>AEEFPVPNGFESAYREVDGVKLHYVKGGQGPLVMLVHGFGQTWYEWHQLMPELAKRFTVIAPDLPGLGQSEPPKTGYSGEQVAVYLHKLARQFSPDRPFDLVAHDIGIWNTYPMVVKNQADIARLVYMEAPIPDARIYRFPAFTAQGESLVWAFSFFAADDRLAETLIAGKERFFLEHFIKSHASNTEVFSERLLDLYARSYAKPHSLNASFEYYRALNESVRQNAELAKTRLQMPTMTLAGGGHGGMGTFQLEQMKAYAE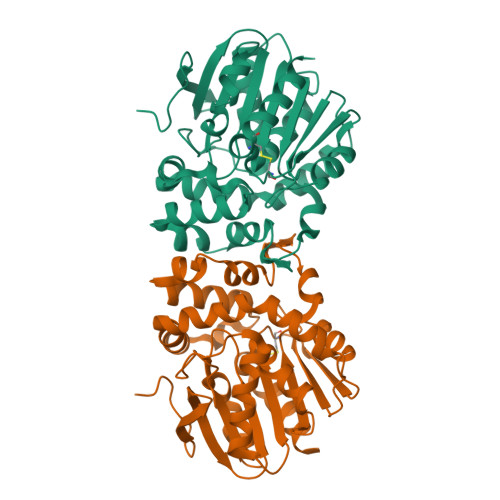DVEGHVLPGCGHWLPEECAAPMNRLVIDFLSRGRHHHHHH[4x]> SSMIPLTPLFSRYKDSYLLYSFRLIDLLRASKSAHLTKLLSSQATYLYHFACLMKYKDIQKYEVQQLIEWAINASPDMDLQQFRIEFMDKTTELNLRSCQPKSFTYTFTTIWDTMHFLSLIIDDMVYTRDKSSLDFVMQQLKTMKVLFYNVFFILQCAMCRDHYMNVKGFLIYHIELIEIALDKEKYGTDITFVDSYQQETAGADAAAVSNNMLMKNLMAYVIMTFHNHVNDYKWIQRN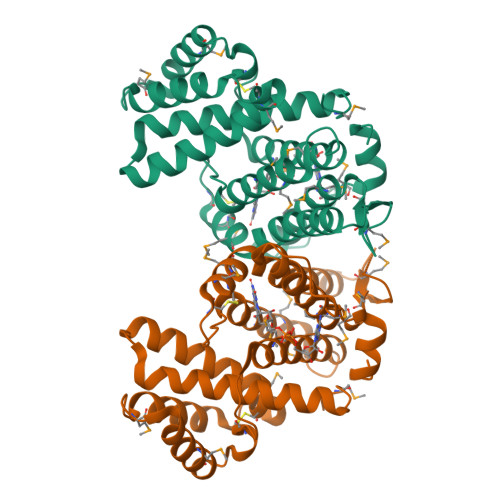QKPPAHYERMTWGEYKKLLNLQHHHHHH The bacteriophage T7, Escherichia coli podophage, has been employed as a model for the investigation of the DNA packaging and delivery mechanism among tailed phages and related dsDNA viruses. The tail, connected to a unique vertex of the head by the dodecameric portal gp8, consists of the dodecameric adaptor protein gp11 and the hexameric nozzle protein gp12 (20, 24) surrounded by six trimeric tail fibers gp17 (16, 22, 24). The core is formed by the core proteins gp14, gp15, and gp16; upon virion adsorption onto host membranes or the receptor rough lipopolysaccharide (LPS), these core proteins have been suggested to extend the tail channel and form a trans-envelope channel for genome delivery into the infected cell. In this study, using a 300 kV cryo-electron microscopy (cryo-EM) and defocus refinement with Z-height correction, we provided improved structures of core proteins at a resolution of 3 Å, the portal–tail complex in mature T7 at a resolution of 2.7 Å, and the portal–tail complex in LPS-induced DNA-ejected T7 at a resolution of 3.5 Å.

We also reconstructed an asymmetric structure of the DNA-ejected T7 complexed with LPS at a resolution of 8.2 Å and the local structure of the portal–tail complex at a resolution of 3.5 Å. Compared with the tail structure of the mature T7, the hexameric tail nozzle of the DNA-ejected T7 undergoes conformational changes, leading to the opening of the tail channel. Hairpin A of one gp12 molecule is close to hairpin B of the adjacent gp12 molecule. By contrast, in DNA-ejected T7, hairpin A of each gp12 molecule rotates almost 90°, leading to the formation of an extended gap for the attachment of the gp14–gp6.7 complex (described below) in the tail channel. Six copies of gp14 (residues 25–143) and twelve copies of gp6.7 (residues) were resolved in the extended channel in the DNA-ejected T7. Each gp14 molecule consists of two antiparallel α-helices connected by a short loop. We resolved two conformers of gp6.7 (conformer A residues 11–41, and conformer B, residues 11–59) in DNA-ejected T7. Moreover, each short α-helix of gp6.7 binds to the turn of the two antiparallel α-helices of gp14, forming a three-helix bundle, and each long loop of gp6.7 connects the cleft between two adjacent gp14 molecules. Six copies of conformer B of gp6.7 are located outside the channel, staying in the opposite direction along the channel compared with the conformer A. Moreover, each short helix α1 binds to the distal end of the two antiparallel α-helices, forming a three-helix bundle, and helix α2 binds to the interface of two adjacent nozzle proteins of gp12 and the turn of the antiparallel α-helices of gp14. The gp14–gp6.7 complex embedded in the open nozzle extends the tail channel, with the distal end of this channel connecting to LPS.

>[6x]MCWAAAIPIAISGAQAISGQNAQAKMIAAQTAAGRRQAMEIMRQTNIQNADLSLQARSKLEEASAELTSQNMQKVQAIGSIRAAIGESMLEGSSMDRIKRVTEGQFIREANMVTENYRRDYQAIFAQQLGGTQSAASQIDEIYKSEQKQKSKLQMVLDPLAIMGSSAASAYASGAFDSKSTTKAPIVAAKGTKTGR;>[12x]MCFSPKIKTPKMDTNQIRAVEPAPLTQEVSSVEFGGSSDETDTEGTEVSGRKGLKVERDDSVAKSKASGNGSARMKSSIRKSAFGGKK;>[12x]MAEKRTGLAEDGAKSVYERLKNDRAPYETRAQNCAQYTIPSLFPKDSDNASTDYQTPWQAVGARGLNNLASKLMLALFPMQTWMRLTISEYEAKQLLSDPDGLAKVDEGLSMVERIIMNYIESNSYRVTLFEALKQLVVAGNVLLYLPEPEGSNYNPMKLYRLSSYVVQRDAFGNVLQMVTRDQIAFGALPEDIRKAVEGQGGEKKADETIDVYTHIYLDEDSGEYLRYEEVEGMEVQGSDGTYPKEACPYIPIRMVRLDGESYGRSYIEEYLGDLRSLENLQEAIVKMSMISSKVIGLVNPAGITQPRRLTKAQTGDFVTGRPEDISFLQLEKQADFTVAKAVSDAIEARLSFAFMLNSAVQRTGERVTAEEIRYVASELEDTLGGVYSILSQELQLPLVRVLLKQLQATQQIPELPKEAVEPTISTGLEAIGRGQDLDKLERCVTAWAALAPMRDDPDINLAMIKLRIANAIGIDTSGILLTEEQKQQKMAQQSMQMGMDNGAAALAQGMAAQATASPEAMAAAADSVGLQPGI;>MRSYDMNVETAAELSAVNDILASIGEPPVSTLEGDANADAANARRILNKINRQIQSRGWTFNIEEGITLLPDVYSNLIVYSDDYLSLMSTSGQSIYVNRGGYVYDRTSQSDRFDSGITVNIIRLRDYDEMPECFRYWIVTKASRQFNNRFFGAPEVEGVLQEEEDEARRLCMEYEMDYGGYNMLDGDAFTSGLLTR[12x];>[18x]MANVIKTVLTYQLDGSNRDFNIPFEYLARKFVVVTLIGVDRKVLTINTDYRFATRTTISLTKAWGPADGYTTIELRRVTSTTDRLVDFTDGSILRAYDLNVAQIQTMHVAEEARDLTTDTIGVNNDGHLDARGRRIVNLANAVDDRDAVPFGQLKTMNQNSWQARNEALQFRNEAETFRNQAEGFKNESSTNATNTKQWRDETKGFRDEAKRFKNTAGQYATSAGNSASAAHQSEVNAENSATASANSAHLAEQQADRAEREADKLENYNGLAGAIDKVDGTNVYWKGNIHANGRLYMTTNGFDCGQYQQFFGGVTNRYSVMEWGDENGWLMYVQRREWTTAIGGNIQLVVNGQIITQGGAMTGQLKLQNGHVLQLESASDKAHYILSKDGNRNNWYIGRGSDNNNDCTFHSYVHGTTLTLKQDYAVVNKHFHVGQAVVATDGNIQGTKWGGKWLDAYLRDSFVAKSKAWTQVWSGSAGGGVSVTVSQDLRFRNIWIKCANNSWNFFRTGPDGIYFIASDGGWLRFQIHSNGLGFKNIADSRSVPNAIMVENE;>MALISQSIKNLKGGISQQPDILRYPDQGSRQVNGWSSETEGLQKRPPLVFLNTLGDNGALGQAPYIHLINRDEHEQYYAVFTGSGIRVFDLSGNEKQVRYPNGSNYIKTANPRNDLRMVTVADYTFIVNRNVVAQKNTKSVNLPNYNPNQDGLINVRGGQYGRELIVHINGKDVAKYKIPDGSQPEHVNNTDAQWLAEELAKQMRTNLSDWTVNVGQGFIHVTAPSGQQIDSFTTKDGYADQLINPVTHYAQSFSKLPPNAPNGYMVKIVGDASKSADQYYVRYDAERKVWTETLGWNTEDQVLWETMPHALVRAADGNFDFKWLEWSPKSCGDVDTNPWPSFVGSSINDVFFFRNRLGFLSGENIILSRTAKYFNFYPASIANLSDDDPIDVAVSTNRIAILKYAVPFSEELLIWSDEAQFVLTASGTLTSKSVELNLTTQFDVQDRARPFGIGRNVYFASPRSSFTSIHRYYAVQDVSSVKNAEDITSHVPNYIPNGVFSICGSGTENFCSVLSHGDPSKIFMYKFLYLNEELRQQSWSHWDFGENVQVLACQSISSDMYVILRNEFNTFLARISFTKNAIDLQGEPYRAFMDMKIRYTIPSGTYNDDTFTTSIHIPTIYGANFGRGKITVLEPDGKITVFEQPTAGWNSDPWLRLSGNLEGRMVYIGFNINFVYEFSKFLIKQTADDGSTSTEDIGRLQLRRAWVNYENSGTFDIYVENQSSNWKYTMAGARLGSNTLRAGRLNLGTGQYRFPVVGNAKFNTVYILSDETTPLNIIGCGWEGNYLRRSSGI[6x]>MKRHHHHHHGSGDLVAWNKENDRRTLWTTPDPEANCKVSEEKDSKLTLVLTKCGSQILASVSLLVVKGKFANINNKTNPGEDYKKFSVKLLFDANGKLLTGSSLDGNYWNYKNKDSVIGSPYENAVPFMPNSTAYPKIINNGTANPEDKKSAAKKTIVTNVYLGGDAAKPVATTISFNKETESNCVYSITFDFAWNKTYKNVPFDSSSLTFSYIAQDAEDKNE[6x]

Here, we investigated HAdV-D49, which previously has been studied for vaccine and vascular gene transfer applications. Here, we investigate the tropism of HAdV-D49, focusing on the fiber knob protein as the major mediator of cellular attachment and evaluate the potential utility of a pseudotyped HAdV-C5/D49K vector to infect a range of cancer cell lines. Structurally and biologically we demonstrate that HAdV-D49 knob protein is unable to engage CD46, while potential interaction with coxsackievirus and adenovirus receptor (CAR) is extremely limited by extension of the DG loop. HAdV-C5/D49K represents a highly efficient gene transfer vehicle that is not restricted by any known adenovirus tropism.

We also used SPR to further probe the binding affinity of HAdV-D49K, and a mutant version, HAdV-D49.KO1.K, for CD46 and CAR. This HAdV-D49.KO1.K mutant, harbors the KO1 mutations S408E and P409A in the fiber knob AB loop, previously shown to ablate CAR binding in HAdV-C5K. As predicted, we did not observe binding between either fiber knob protein and CD46. However, we did observe HAdV-D49K binding to CAR with a detectable 0.19 μM affinity which was ablated by the KO1 mutation. However, no IC50 could be derived by using HAdV-D49K to block CD46 on CHO-BC1 cells, where HAdV-D49K was unable to achieve >20% inhibition of antibody binding, suggesting weak or incidental CD46 interactions. Therefore, these data support the findings from SPR and transduction experiments that HAdV-D49K may bind CAR with low affinity but does not bind CD46. We investigated the transduction efficiency of HAdV-C5/D30K compared to HAdV-C5/D49K, HAdV-C5, HAdV-C5.KO1, and HAdV-C5/D49.KO1.K in CHO-CAR and CHO-K1 cells. HAdV-C5 infected CHO-CAR cells efficiently, while the CAR-binding ablated KO1 mutant did not, and HAdV-C5/49K and the corresponding mutant HAdV-C5/49KO1.K infected CHO-CAR cells with similar efficiency, as observed for HAdV-C5/D49K in Fig. 1A. In CHO-K1 cells, HAdV-C5/D49K and the KO1 mutant were the only viruses that achieved efficient transduction. In support of this, we show that a mutant vector, HAdV-C5/D49.KO1.K, containing mutations within the fiber knob domain which ablate CAR affinity, retained the ability to efficiently transduce cells in the absence of any detectable binding to CAR. We demonstrate that the HAdV-D49 fiber knob has a weak affinity for CAR, although it is not dependent upon this interaction to mediate efficient cell entry, and in fact the presence of CAR may inhibit cellular transduction.>[2x]GKTITGVFNSFNSLTWSNAATYNYKGPGTPTWNAVLGWSLDGTSASPGDTFTLNMPCVFKFTTSQTSVD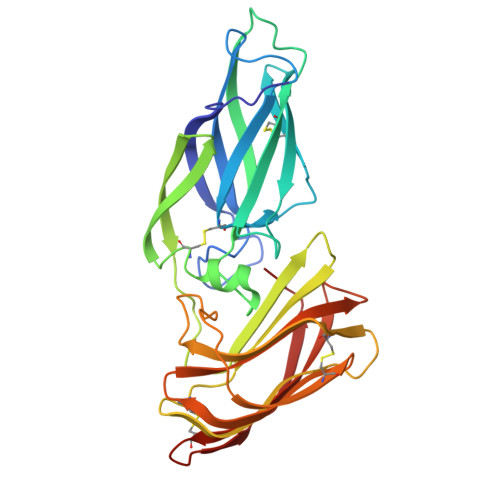LTAHGVKYATCQFQAGEEFMTFSTLTCTVSNTLTPSIKALGTVTLPLAFNVGGTGSSVDLEDSKCFTAGTNTVTFNDGGKKISINVDFERSNVDPKGYLTDSRVIPSLNKVSTLFVAPQCANGYTSGTMGFANTYGDVQIDCSNIHVGITKGLNDWNYPVSSESFSYTKTCSSNGIFITYKNVPAGYRPFVDAYISATDVNSYTLSYANEYTCAGGYWQRAPFTLRWTGYR>[2x]GPGHMAQVAGAALSQAGWYLSDEGIEACT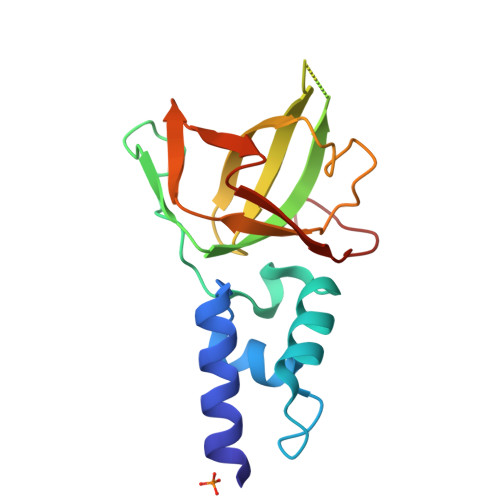SSPDKVNVNDIILIALNTDLRTIGKKFLPSDINSGKVEKLEGPCVLQIQKIRNVAAPKDNEESQAAPRMLRLQMTDGHISCTAVEFSYMSKISLNTPPGTKVKLSGIVDIKNGFLLLNDSNTTVLGGEVEHLIEKW> KPGDVDGNG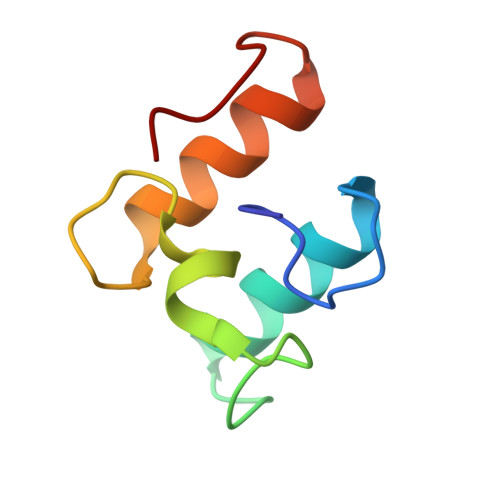SININDFALMRNYLLGNLKDFPAEDDIKAGDLNGDKSINSLDFAIMRMYLLGMITKFSV>[6x]SMAGKEIQTPDQAEAFVAKVFDVLDSYDYTRFGEVLSTDLKYEGGLQKTSGLDNFINDIKASTQRMPGLQTSHSRYRTELTAEGTIYSEGHSNASLESNPGKVVTVPMIGVFKLDSEDGK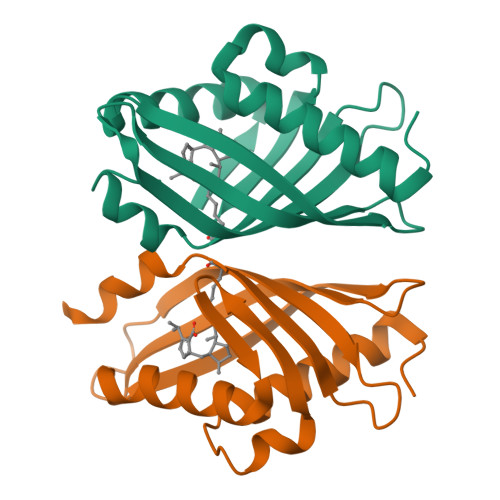IKEMRIYKDRLPFLALHQALPGMKANN> XAPY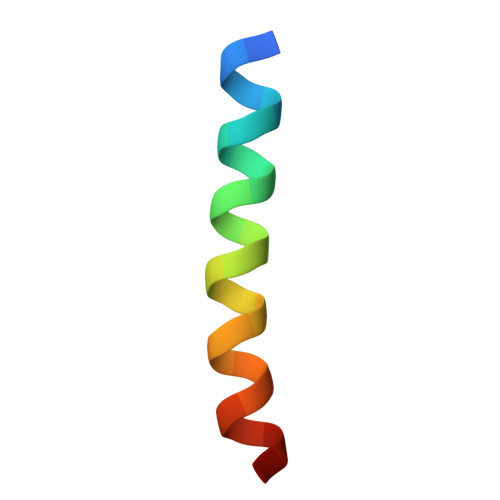LEQVARTLRKIGEEINEALRX> MGTTTVGLVCKDGVVMATEKRATMGNFIASKAAKKIYQIADRMAMTTAGSVGDAQFLARIIKIEANLYEIRRERKPTVRAIATLTSNLLNSYRYFPYLVQLLIGGIDSEGKSIYSIDPIGGAIE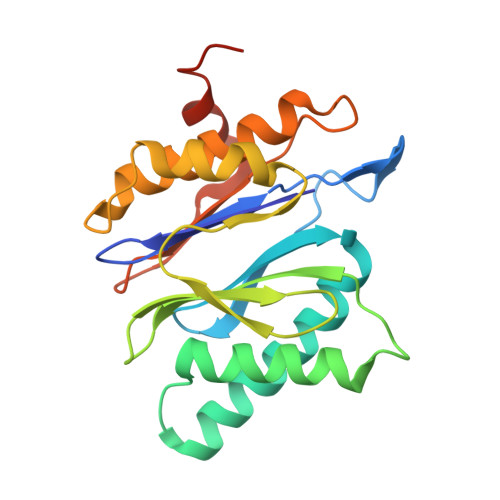EKDIVATGSGSLTAYGVLEDRFTPEIGVDEAVELAVRAIYSAMKRDSASGDGIDVVKITEDEFYQYSPEEVEQILAKFRKHHHHHH> AATATLPTTASSSTAVASSQLDQLANFAYNVTTDSVAGG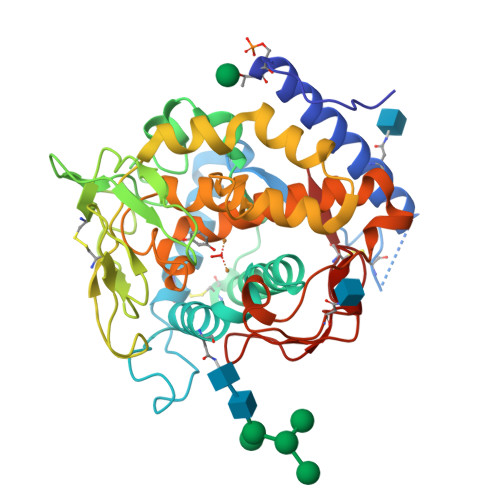SESKRGGCTLQNLRVRRDWRAFSKTQKKDYINSVLCLQKLPSRTPAHLAPGARTRYDDFVATHINQTQIIHYTGTFLAWHRYFIYEFEQALRDECSYTGDYPYWNWGADADNMEKSQVFDGSETSMSGNGEYIPNQGDIKLLLGNYPAIDLPPGSGGGCVTSGPFKDYKLNLGPAALSLPGGNMTAAANPLTYNPRCMKRSLTTEILQRYNTFPKIVELILDSDDIWDFQMTMQGVPGSGSIGVHGGGHYSMGGDPGRDVYVSPGDTAFWLHHGMIDRVWWIWQNLDLRKRQNAISGTGTFMNNPASPNTTLDTVIDLGYANGGPIAMRDLMSTTAGPFCYVYL> MERLWKDIKRDWLLYAMLLPTIIWFLIFLYKPMIGLQMAFKQYSAWKGIAGSPWIGFDHFVTLFQSEQFIRAIKNTLTLSGLSLLFGFPMPILLALMINEVYSKGYRKAVQTIVYLPHFISIVIVAGLVVTFLSPSTGVVNNMLSWIGLDRVYFLTQPEWFRPIYISSNIWKEAGFDSIVYLAAIMSINPALYESAQVDGATRWQMITRITLPCIVPTIAVLLVIRLGHILEVGFEYIILLYQPTTYETADVISTYIYRLGLQGARYDIATAAGIFNAVVALVIVLFANHMSRRITKTGVF;> MLATPFYSRSDRIFGIVNAVLLGIFALCALYPIIYIFSMSISSGAAVTQGRVFLLPVDIDFSAYGRVLHDKLFWTSYANTIFYTVFGVVTSLIFIVPGAYALSKPRIRGRRVFGFIIAFTMWFNAGMIPFFLNMRDLGLLDNRFGILIGFACNAFNIILMRNYFESISASFEEAARMDGANDLQILWKVYIPLAKPALATITLLCAISRWNGYFWAMVLLRAEEKIPLQVYLKKTIVDLNVNEEFAGALLTNSYSMETVVGAIIVMSIIPVIIVYPVVQKYFTKGVMLGGVKELEHHHHHHHHHH;> MKKMMLSVAAVATLMAFAAPVATAKEATWVTDKPLTLKIHMHFRDKWVWDENWPVAKESFRLTNVKLQSVANKAATNSQEQFNLMMASGDLPDVVGGDNLKDKFIQYGQEGAFVPLNKLIDQYAPHIKAFFKSHPEVERAIKAPDGNIYFIPYVPDGVVARGYFIREDWLKKLNLKPPQNIDELYTVLKAFKEKDPNGNGKADEVPFIDRHPDEVFRLVNFWGARSSGSDNYMDFYIDNGRVKHPWAETAFRDGMKHVAQWYKEGLIDKEIFTRKARAREQMFGGNLGGFTHDWFASTMTFNEGLAKTVPGFKLIPIAPPTNSKGQRWEEDSRQKVRPDGWAITVKNKNPVETIKFFDFYFSRPGRDISNFGVPGVTYDIKNGKAVFKDSVLKSPQPVNNQLYDMGAQIPIGFWQDYDYERQWTTPEAQAGIDMY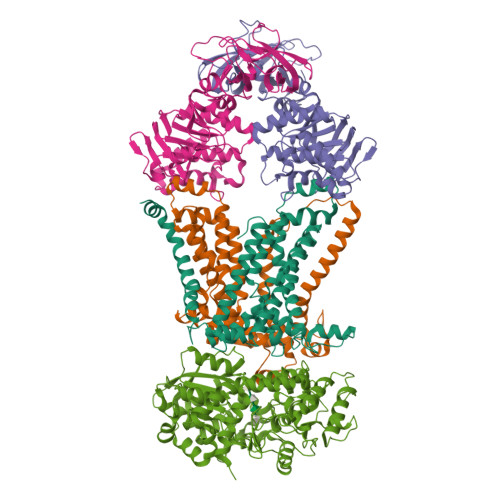VKGKYVMPGFEGVNMTREERAIYDKYWADVRTYMYEMGQAWVMGTKDVDKTWDEYQRQLKLRGLYQVLQMMQQAYDRQYKN;>MVASVSIQNVVKRYDKTTVVHGVSLDIEPGEFVVLVGPSGCGKSTTLRMVAGLEEISGGTIRIDGRVINDLAPKDRDVAMVFQNYALYPHLNVRDNISFGLRLKRTKKSVIDAAVKTAADILGLQPLLERKPSDLSGGQRQRVAMGRAIVRDPKVFLFDQPLSNLDAKLRTQMRAEIKRLHQRLGTTVIYVTHDQVEAMTLADRIVVMRDGLIEQIGKPMDLFLHPANTFVASFIGSPPMNLMPARIAVDSTQHVELNGGNRISLLPRAGTHLAPGQEVVFGIRPEDVTLDGVEGSERAQIKATVDIVEPLGSESILHATVGDHSLVVKVGGLNEVHPGDPVTLHVDLTRVHLFDAQSQASIY[2x]>MKEKEFQSKPLLTKRERE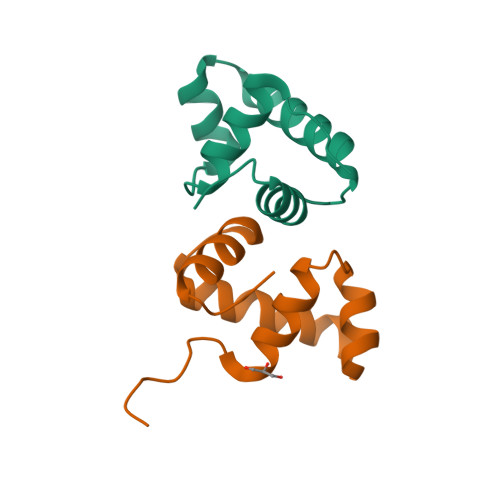VFELLVQDKTTKEIASELFISEKTVRNHISNAMQKLGVKGRSQAVVELLRMGELEL[6x]>[2x]HHHHHHGCMSGRKPIIGVMGPGKADTAENQLVMANELGKQIATHGWILLTGGR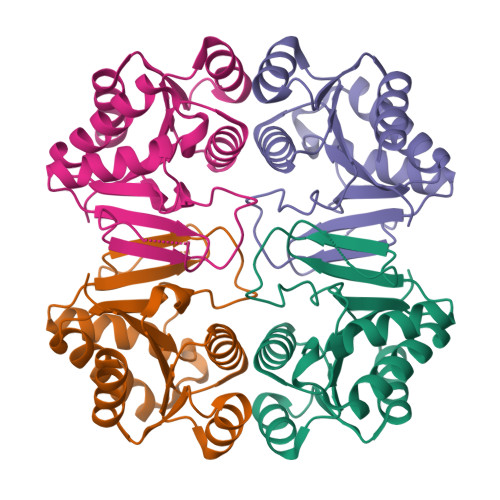SLGVMHEAMKGAKEAGGTTIGVLPGPDTSEISDAVDIPIVTGLGSARDNINALSSNVLVAVGMGPGTAAEVALALKAKKPVVLLGTQPEAEKFFTSLDAGLVHVAADVAGAIAAVKQLLAKLN>[2x]MSRQASRLDAKKVNSEFLTLTYGALVTQMLRDFENAEDVNKQLERIGYNMGMRLIEDFLARTSAPRCLEMRETADRIQQAFRIYLNIQPTISNWSPASDEFSLVFDSNPLTEFVELPPDLTNLRYSAILSGCIRGALEMVQLEVQCWFVQDQLKGDNVTELRVKFVRRLEEVIPAGEDLEVLFQGPVASWSHPQFEKGAV;> MSEEILFDCLHAEIVNYCLDSNKEHDLATLEYIGFTTGYRLIERLTREVSRFKDELETMKFICTDFWMLIYKKQVDNLRTNNHGMYVVQDKAFRFLTRISPGTKQLEHAPKFVAFTCGLVRGALSNLGINSTVTAEVQSIPACKFHIEVNRN;> MTIFNLYIFDKFGTLLHYAEWNRTKKSGITREEEAKLTYGMLFSIKSFVSKISPHDPKEGFLYYKTNRYALHYLETPSGLKFVLNTDTTAINVKELLQQLYAKVWVEFVVRDPLWTPGTVVTSELFQSKLDEFVRQSPIFGIRNI;> MIIYGVYIVSKSGGLIFNLDNNVPRIEHEKTFTYPLDLVLDYDSKKVSVSFNRKDGINVGHVLVAVNGMPVNGVTLDDGRDVRTTLDAPENYPINLKFSRPKMTTNEKIFLASMFYPLFAIASQLSPEPKSSGIEILEADTFTLHCFQTLTGIKFIII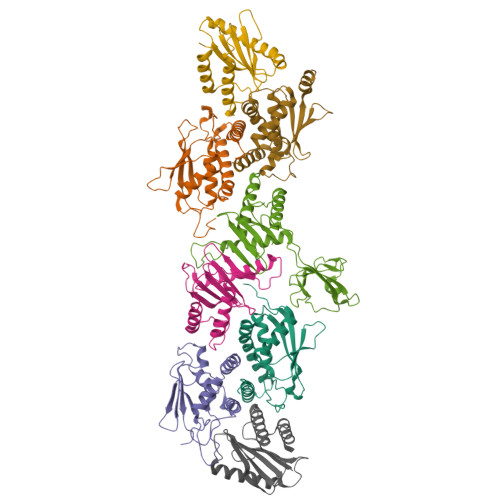SETGLNGIDLLLRKVYELYSDYVLKNPFYSLEMPIRCELFDNKLQELLAQVEKTGISNIDK;> MSTYYFVIVGQNDNPIYEKEFSTVNKELRKEDHRHLTQFIAHAALDLVDEHKWKTANMQLKSIDRFNQWFVSAFITASQIRFIIVHDNKNDEGIKNFFNEMYDTYIKNSMNAFYRINTPIKSPMFEKKSEIFGRKYLLS;> MEKLEALKISSMRPRSNILDRPLSKGKTEVSQSIVALLFSEIVQYSQSRVFTVPELQTRLHDLGQDVGTRIIDLYFVRERSSKRETKLTQMLLFVKTTVWKNLFGKEAEKLEHANDDERTYYIIEKEPLVNTFISVPKDKGSLNCANFTAGIVEAVLTNCGFPCKVTAHWHKGTTYMVKFEDFVIARDKQMEEK;> MAFCIAVIGKDNAPLYLTTSDMEQELELQYHVNAALDVVEEKCLIGKGAPESKELYLGLLYSTENHKIYGFVTNTRVKFIVVIDSSNVALRENEVRAIFRNLHLLYTDAICNPFYIPGESLTSKKFDRAVQKLMSGTA> ARDPKHDILFEPIQIGPKTLRNRFYQVPHCIGAGSDKPGFQSAHRSVKAEGGWAALNTEYCSINPESDDTHRLSARIWDEGDVRNLKAMTDEVHKYGALAGVELWYGGAHAPNMESRATPRGPSQYASEFETLSYCKEMDLSDIAQVQQFYVDAAKRSRDAGFDIVYVYGAHSY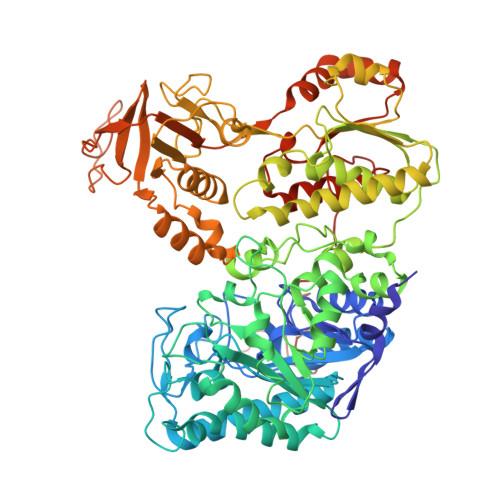LPLQFLNPYYNKRTDKYGGSLENRARFWLETLEKVKHAVGSDCAIATRFGVDTVYGPGQIEAEVDGQKFVEMADSLVDMWDITIGDIAEWGEDAGPSRFYQQGHTIPWVKLVKQVSKKPVLGVGRYTDPEKMIEIVTKGYADIIGCARPSIADPFLPQKVEQGRYDDIRVCIGCNVCISRWEIGGPPMICTQNATAGEEYRRGWHPEKFRQTKNKDSVLIVGAGPSGSEAARVLMESGYTVHLTDTAEKIGGHLNQVAALPGLGEWSYHRDYRETQITKLLKKNKESQLALGQKPMTADDVLQYGADKVIIATGARWNTDGTNCLTHDPIPGADASLPDQLTPEQVMDGKKKIGKRVVILNADTYFMAPSLAEKLATAGHEVTIVSGVHLANYMHFTLEYPNMMRRLHELHVEELGDHFCSRIEPGRMEIYNIWGDGSKRTYRGPGVSPRDANTSHRWIEFDSLVLVTGRHSECTLWNELKARESEWAENDIKGIYLIGDAEAPRLIADATFTGHRVAREIEEANPQIAIPYKRETIAWGTPHMPGGNFKIEYKV> GMADKTGTPHPLTEPGVWIERIGGRVFPPHLPALFLDRDGTINVDTDYPSDPAEIVLRPQMLPAIATANRAGIPVVVVTNQSGIARGYFGWSAFAAVNGRVLELLREEGVFVDMVLACAYHEAGVGPLAIPDHPMRKPNPGMLVEAGKRLALDLQRSLIVGDKLADMQ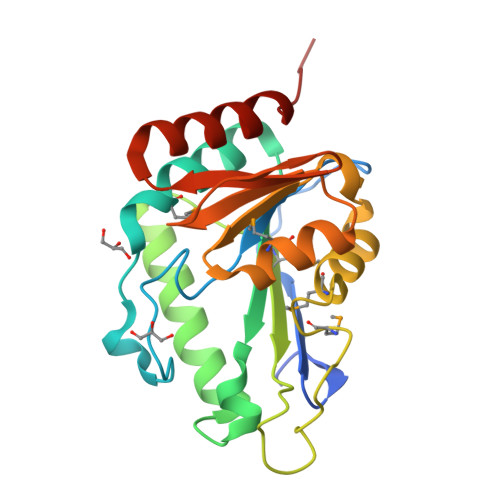AGKRAGLAQGWLVDGEAAVQPGFAIRPLRDSSELGDLLAAIETLGRDNRS Cobamides (Cbas) are coenzymes used by cells across all domains of life, but de novo synthesis is only found in some bacteria and archaea. Base activation is catalyzed by a phosphoribosyltransferase (PRTase). To gain insights into the mechanism of base activation by the PRTase from Methanocaldococcus jannaschii (MjCobT), we solved crystal structures of the enzyme in complex with substrate and products. The protein fold consists of an eight-stranded mostly parallel β-sheet with connecting α-helices on both sides where the substrate binding pocket is built from the connecting loops and resides at the end of the C-terminal end of β-strands.

MjCobT was crystallized in the presence of DMB at pH 7.0 and gave a crystal lattice that contained two protein subunits per asymmetric units. These crystals were soaked in 1 mM NaMN and a nucleotide base overnight prior to freezing. During that time the enzyme catalyzed a transferase reaction. The contents of the two active sites are different. One subunit contains NaMN, whereas the second includes α-RP and nicotinic acid. This provides an opportunity to observe substrate and product in the same crystal lattice. NaMN lies at the base of the active site for chain A where there are extensive hydrogen bonding interactions with the phosphoryl moiety, and specific interactions with the ribose 2′ and 3′-oxygens and the carboxylate group of NaMN. The coordination of the ribose, phosphate, and nicotinic acid moieties in the active site that complexed α-RP is very similar to what was observed for NaMN. However, there are additional hydrogen bonds between O2’ of the ribose and Oγ1 and Oγ2 of Glu 150. There is a hydrogen bond between an imidazole nitrogen of DMB and Oγ of Asp 52 that fulfills the hydrogen bonding potential of the benzimidazole ring.

>MSIIAINENGFLDKIKGRNPLFTCVISSIETTLSIPISGVHRDVIKYTPSADVELVFYGKSLTLKTPPIDATGSPTPATITRACVELKNIKNLHIDAGAFVKPKIPFIEIDEKPTGRIEEGKAMNNSKELYMKGYLLGKNLDAELLIVGESVPGGTTTALGVLLGLGYDAEGKVSSGSINNPHELKIKVVREGLKKAGINEKSSVFDVLNAVGDKMMPVVAGLAISFAERNKPVILAGGTQMSAVLAVIKEINKKVLDKNLIAIGTTEFVLNDKKGDLKGIVEQIGNVPVLASKFYFEKAKIEGLKNYCKGSVKEGVGAGGIAVYSIVNDLEPTKIREFIENKFYEWYKE[2x]FAM111A (FAM111 trypsin-like peptidase A) is a serine protease involved in multiple cellular processes including antiviral defense and DNA replication. FAM111A contains a serine protease domain (SPD) with a conserved catalytic triad (His385, Asp439, and Ser541). The FAM111A SPD belongs to the S1 family of serine peptidases, which includes chymotrypsin, in the MEROPS database. Here, we show that FAM111A is a dimerization-dependent protease containing a narrow, recessed active site that cleaves substrates with a chymotrypsin-like specificity.

Therefore, to generate a mutant SPD that would crystalize without forming the α1 dimer interface even at the very high concentrations used for crystallization, we truncated the N-terminal SPD to remove two-thirds of the dimer interface and included an engineered V347D mutation to create a construct that we have named mini-SPD. The mini-SPD crystallized with two polypeptide chains present in the asymmetric unit. Although helix α1 is still present and visible in the electron density map, the dimerization interface observed in the full SPD dimer structure is noticeably absent. Overall, the mini-SPD and SPD dimer structures possess a significant degree of similarity with an overall RMSD value of 0.5 Å, but with some small yet impactful differences. The catalytic triad Asp-His-Ser (in this construct the catalytic Ser541 was retained as wildtype) is unchanged, which is expected as they are anchored on the rigid beta-barrel domain. In contrast, several disordered regions were noted in the mini-SPD where some of the residues comprising the dimerization interface, several surface-exposed loops, and the oxyanion hole are altered. Residues 413-422 that form a part of the loop L4 between β4 and β5 were disordered and not observed in the mini-SPD. Another region adjoining the β6-β7 loop (Loop L6, residues 474-480) is also disordered in one chain and altered compared to the dimeric SPD in the other chain. The differences observed between the two chains of the mini-SPD structure and the dimeric SPD as well as the higher B-factors observed for residues 536–538 encompassing the oxyanion hole and S1 pocket indicate that the monomeric SPD is more disordered. This suggests that dimerization of the SPD is associated with a disorder-to-order transition that supports the oxyanion hole residues in the conformation that is competent for catalysis.

>GHMKVDKLLVRLSDSVGYLFWDSATTGYATCFVFKGLFILTCRHVIDSIVGDGIEPSKWATIIGQCVRVTFGYEELKDKETNYFFVEPWFEIHNEELDYAVLKLKENGQQVPMELYNGITPVPLSGLIHIIGHPYGEKKQIDACAVIPQGQRAKKCQERVQSKKAESPEYVHMYTQRSFQKIVHNPDVITYDTEFFFGASGSPVFDSKGSLVAMHAAGFAYTYQNETRSIIEFGSTMESILLDIKQRHKPWYEEVFVNQQDVEMMSDEDL[2x]>[2x]NSKDSIVNDDDDSTSEVDAIPDSTNPSGSFPSVEYDVFLSFRGPDTRKQFTDFLYHFLCYYKIHTFRDDDELRKGKEIGPNLLRAIDQSKIYVPII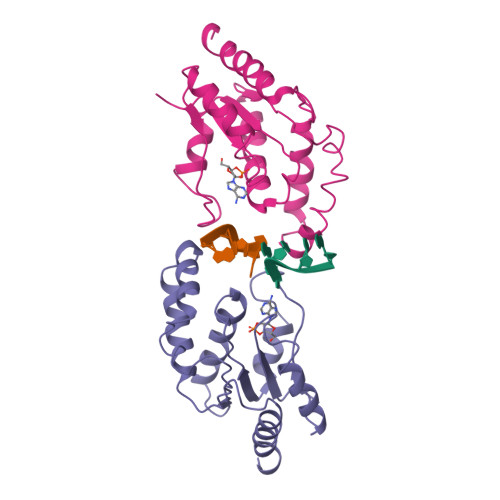SSGYADSKWCLMELAEIVRRQEEDPRRIILPIFYMVDPSDVRHQTGCYKKAFRKHANKFDGQTIQNWKDALKKVGDLKGWHIGKDDEQGAIADKVSADIWSHISKENL(2R)-2,3-dihydroxypropyl (2S)-2,3-dihydroxypropyl hydrogen phosphate | C6 H15 O8 P | 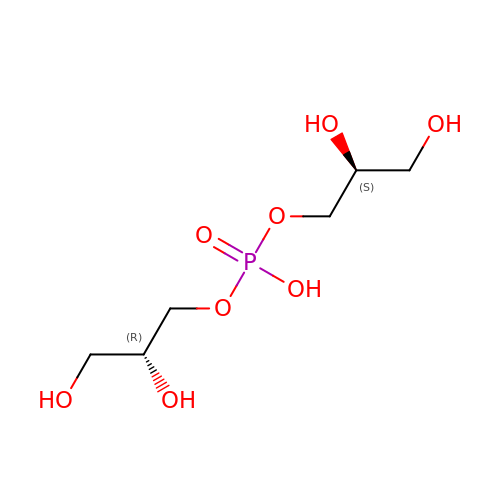LLCSXHMJULHSJN-OLQVQODUSA-N>MKIGIIAAMPEELAYLVQHLDNTQEQVVLGNTYHTGTIASHEVVLVESGIGKVMSAMSVAILADHFQVDALINTGSAGAVAEGIAVGDVVIADKLAYHDVDVTAFGYAYGQMAQQPLYFESDKTFVAQIQESLSQLDQNWHLGLIATGDSFVAG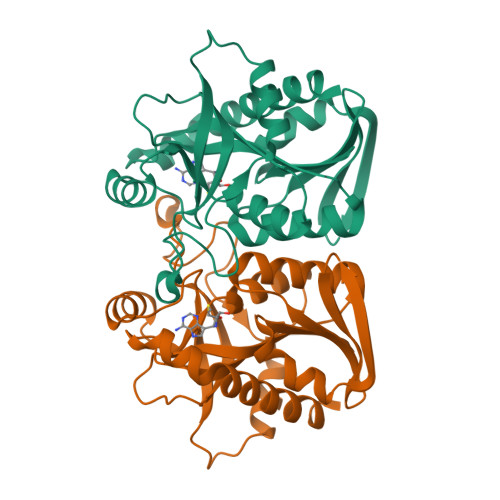NDKIEAIKSHFPEVLAVEMEGAAIAQAAHTLNLPVLVIRAMSDNANHEANIFFDEFIIEAGRRSAQVLLAFLKALD[6x]>[4x]GPGS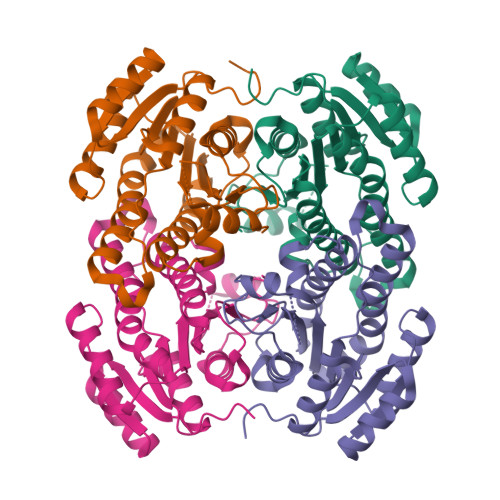MFDLTGRKALVTGATGGLGEAIARALHAQGAIVGLHGTREEKLKELAAELGERIFVFPANLSDREAVKALGQKAEEEMGGVDILVNNAGITRDGLFVRMSDEDWDAVLTVNLTSVFNLTRELTHPMMRRRNGRIINITSIVGVTGNPGQANYCASKAGLIGFSKSLAQEIASRNVTVNCIAPGFIESAMTGKLNEKQKDAIMGNIPMKRMGVGADIAAAVVYLASDEAAYVTGQTLHVNGGMAMI> SKFLDRFRYFKQKGETFADGHGQLLNTNRDWEDGYRQRWQHDKIVRSTHGVNCTGSCSWKIYVKNGLVTWETQQTDYPRTRPDLPNHEPRGCPRGASYSWYLYSANRLKYPMMRKRLMKMWREAKALHSDPVEAWASIIEDADKAKSFKQARGRGGFVRSSWQEVNELIAASNVYTIKNYGPDRVAGFSPIPAMSMVSYASGARYLSLIGGTCLSFYDWYCDLPPASPQTWGEQTDVPESADWYNSSYIIAWGSNVPQTRTPDAHFFTEVRYKGTKTVAVTPDYAEIAKLCDLWLAPKQGTDAAMALAMGHVMLREFHLDNPSQYFTDYVRRYTDMPMLVMLEERDGYYAAGRMLRAADLVDALGQENNPEWKTVAFNTNGEMVAPNGSIGFRWGEKGKWNLEQRDGKTGEETELQLSLLGSQDEIAEVGFPYFGGDGTEHFNKVELENVLLHKLPVKRLQLADGSTALVTTVYDLTLANYGLERGLNDVNCATSYDDVKAYTPAWAEQITGVSRSQIIRIAREFADNADKTHGRSMIIVGAGLNHWYHLDMNYRGLINMLIFCGCVGQSGGGWAHYVGQEKLRPQTGWQPLAFALDWQRPARHMNSTSYFYNHSSQWRYETVTAEELLSPMADKSRYTGHLIDFNVRAERMGWLPSAPQLGTNPLTIAGEAEKAGMNPVDYTVKSLKEGSIRFAAEQPENGKNHPRNLFIWRSNLLGSSGKGHEFMLKYLLGTEHGIQGKDLGQQGGVKPEEVDWQDNGLEGKLDLVVTLDFRLSSTCLYSDIILPTATWYEKDDMNTSDMHPFIHPLSAAVDPAWEAKSDWEIYKAIAKKFSEVCVGHLGKETDIVTLPIQHDSAAELAQPLDVKDWKKGECDLIPGKTAPHIMVVERDYPATYERFTSIGPLMEKIGNGGKGIAWNTQSEMDLLRKLNYTKAEGPAKGQPMLNTAIDAAEMILTLAPETNGQVAVKAWAALSEFTGRDHTHLALNKEDEKIRFRDIQAQPRKIISSPTWSGLEDEHVSYNAGYTNVHELIPWRTLSGRQQLYQDHQWMRDFGESLLVYRPPIDTRSVKEVIGQKSNGNQEKALNFLTPHQKWGIHSTYSDNLLMLTLGRGGPVVWLSEADAKDLGIADNDWIEVFNSNGALTARAVVSQRVPAGMTMMYHAQERIVNLPGSEITQQRGGIHNSVTRITPKPTHMIGGY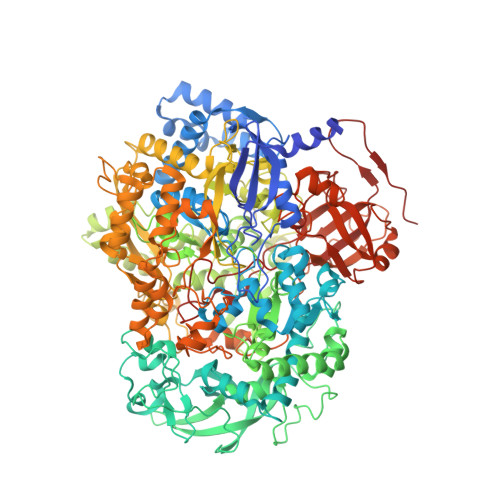AHLAYGFNYYGTVGSNRDEFVVVRKMKNIDWLDGEGNDQVQESVK>MDYKDDDDKLEMPMAQSSCPGSPPDTGDGWEPVLCKGEVNFGGSGKKRSKFVKVPSNVAPSMLFELLLTEWHLPAPNLVVSLVGEERLFAMKSWLRDVLRKGLVK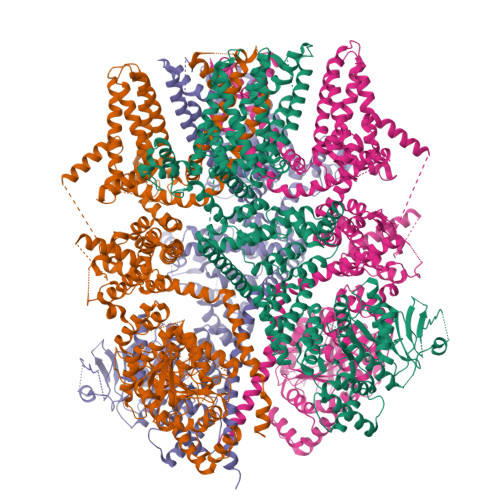AAQSTGAWILTSALHVGLARHVGQAVRDHSLASTSTKVRVVAIGMASLDRILHRQLLDGVQAQEDTPIHYPADEGSTQGPLCPLDSNLSHFILVEPGTLGSGNDGLAELQLSLEKHISQQRTGYGGTSSIQIPVLCLLVNGDPSTLERMSRAVEQAAPWLILAGSGGIADVLAALVGQPHLLVPQVTEKQFREKFPSECFSWEAIVHWTELLQNIAAHPHLLTVYDFEQEGSEDLDTVILKALVKACKSHSRDAQDYLDELKLAVAWDRVDIAKSEIFNGDVEWKSCDLEEVMTDALVSNKPDFVRLFVDSGADMAEFLTYGRLQQLYHSVSPKSLLFELLERKHEEGRLTLAGLGAQQTRELPVGLPAFSLHEVSRVLKDFLHDACRGFYQDGRRMEERGPPKRPAGQKWLPDLSRKSEDPWRDLFLWAVLQNRYEMATYFWAMGREGVAAALAACKIIKEMSHLEKEAEVARTMREAKYEQLALDLFSECYSNSEDRAFALLVRRNHSWSRTTCLHLATEADAKAFFAHDGVQAFLTKIWWGDMATGTPILRLLGAFTCPALIYTNLISFSEDAPQRMDLEDLQEPDSLDMEKSFLCSHGGQLEKLTEAPRAPGDLGPQAAFLLTRWRKFWGAPVTVFLGNVVMYFAFLFLFSYVLLVDFRPPPQGPSGSEVTLYFWVFTLVLEEIRQGFFTNEDTRLVKKFTLYVEDNWNKCDMVAIFLFIVGVTCRMVPSVFEAGRTVLAIDFMVFTLRLIHIFAIHKQLGPKIIIVERMMKDVFFFLFFLSVWLVAYGVTTQALLHPHDGRLEWIFRRVLYRPYLQIFGQIPLDEIDEARVNCSLHPLLLDSSASCPNLYANWLVILLLVTFLLVTNVLLMNLLIAMFSYTFQVVQGNADMFWKFQRYHLIVEYHGRPALAPPFILLSHLSLVLKQVFRKEAQHKQQHLERDLPDPVDQKIITWETVQKENFLSTMEKRRRDSEEEVLRKTAHRVDLIAKYIGGLREQEKRIKCLESQANYCMLLLSSMTDTLAPGGTYSSSQNCGRRSQPASARDREYLEAGLPHSDT[4x]> LSSSITSVTTIDVLSSLFINLFENDLIPQALKDFNKSDDDQFRKLLYKLDLRLFQTISDQMTRDLKDILDINVSNNELCYQLKQVLARKEDL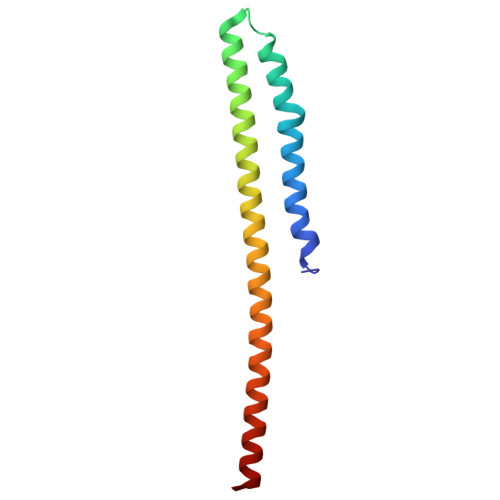NQQIISVRNEIQELK>VVGGLVALRGAHPYIAALYWGHSFCAGSLIAPCWVLTAAHCLQDRPAPEDLTVVLGQERRNHSCEPCQTLAVRSYRLHEAFSPVSYQHDLALLRLQEDADGSCALLSPYVQPVCLPSGAARPSETTLCQVAGWGHQFEGAEEYASFLQEAQVPFLSLERCSAPDVHGSSILPGMLCAGFLEGGTDACQGDSGGPLVCEDQAAERRLTLQGIISWGSGCGDRNKPGVYTDVAYYLAWIREHTVS[2x];>YFAYDRRXLSNNXRNYCG[2x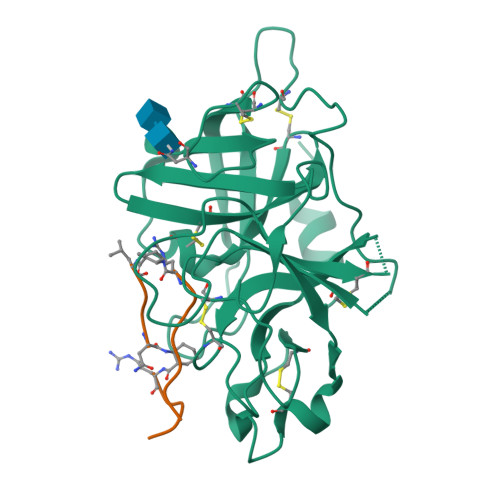]> NDTIASQDTPAKVVIKANKLKDLKDYVDDLKTYNNTYSNVVTVAGEDRIETAIELSSKYYNSDDKNAITDKAVNDIVLVGSTSIVDGLVASPLASEKTAPLLLTSKDKLDSSVKSEIKRVMNLKSDTGINTSKKVYLAGGVNSISKDVENELKNMGLKVTRLSGEDRYETSLAIADEIGLDNDKAFVVGGTGLADAMSIAPVASQLKDGDATPIVVVDGKAKEISDDAKSFLGTSDVDIIGGKNSVSKEIEESIDSATGKTPDRISGDDRQATNAEVLKEDDYFTDGEVVNYFVAKDGSTKEDQLVDALAAAPIAGRFKESPAPIILATDTLSSDQNVAVSKAVP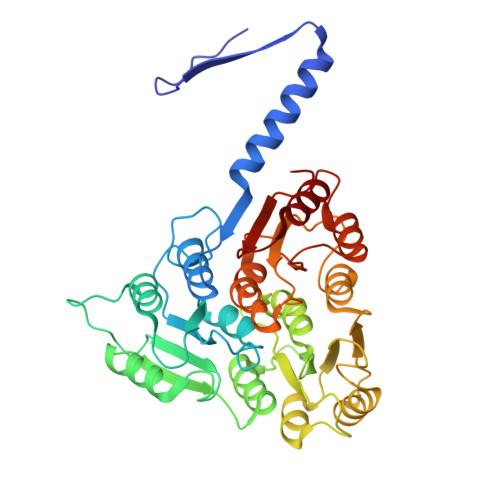KDGGTNLVQVGKGIASSVINKMKDLLDM>MALQEIEFTSHNGRDAIQAWAYEPVGTPTAVVQIIHGLGEHSRRYLHMISALLDAGFVVIADDHAGHGRTAMQSGVWADAGDNAAEVVISDELTLQQQLAGQFDDLPWVVFGHSWGSMIARAMATRPGTRLDGLALCGIVAQPRGFETTLDHKTLAKAMATAPTDPAPEALVAQMFDGFADRLSEDDGPTGWVARSKEVVADHGKDKFNNFGAPMSTRFLQGLADIYAMANGDSFYATMPNIPIVLFAGSEDPAGDFGTGVKA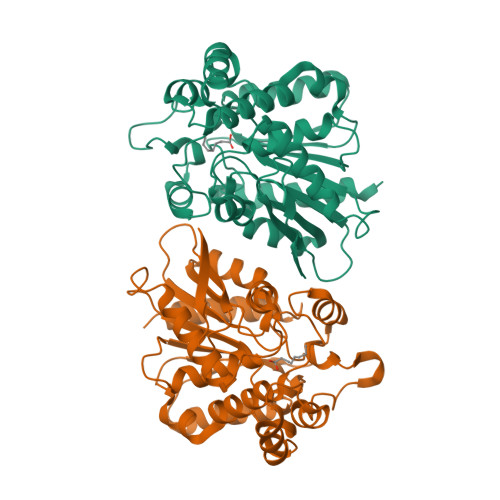VAERLRRDGHNVELHLYDGLRHEVHNEPESRADVESSLVTFVDRVANRRIKRSR[26x]>[2x]GAMGITADKITSFADWYSQVIVKSEMIEYYDISG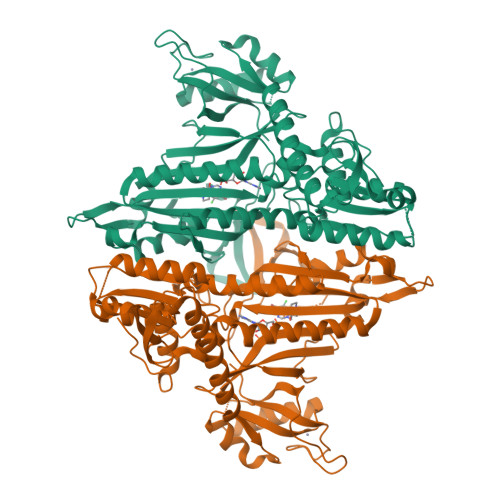CYILRPWSYFIWETIQSVFDQKIKQHDVQNAYFPIFVTQKKLETEKDHVEGFSPEVAWVTKSGKSDLAEPIAIRPTSETIMYPYFAKWIRSHRDLPLKINQWTSIVRWEFKHPTPFIRTREFLWQEGHTAHSTRKEALEMVDIILNEYASIYEDLLATPVVKGTKSENEKFPGGDITKSIEGFIPEIGRAVQAATSHLLGQNFSKMFGVEFEDEKGNKEYAHQTSWGLTTRAIGVMIMTHGDNKGLVLPPKVAPVQVIIIPIIFKTVITEEQKKICNEVECILKKAGVRVKIDDRSNYTPGWKYNHWEVKGVCLRFEVGPRDIEKRSVRVVVRDNMEKMDIPISELESKIPKLLEEFQNRLLFKAKQRQNESIIRVDTFDKVMDTLNQKKMVIAPWCEDVSCEEEIKKETARLSLDNEDNQSMTGAMKSLCIPNDQIFKIEEGKTKCFFCDKLAKKFTLFGRSY> NKDPNEVRS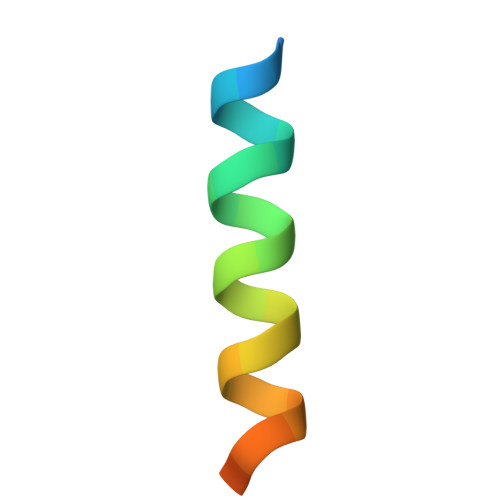FLQDLSQVLARKSQGN>AAAAANHSTQESGFDYEGLIDSELQKKRLDKSYRYFNNINRLAKEFPLAHRQREADKVTVWCSNDYLALSKHPEVLDAMHKTIDKYGCGAGGTRNIAGHNIPTLNLEAELATLHKKEGALVFSSCYVANDAVLSLLGQKMKDLVIFSDELNHASMIVGIKHANVKKHIFKHNDLNELEQLLQSYPKSVPKLIAFESVYSMAGSVADIEKICDLADKYGALTFLDEVHAVGLYGPHGAGVAEHCDFESHRASGIATPKTNDKGGAKTVMDRVDMITGTLGKSFGSVGGYVAASRKLIDWFRSFAPGFIFTTT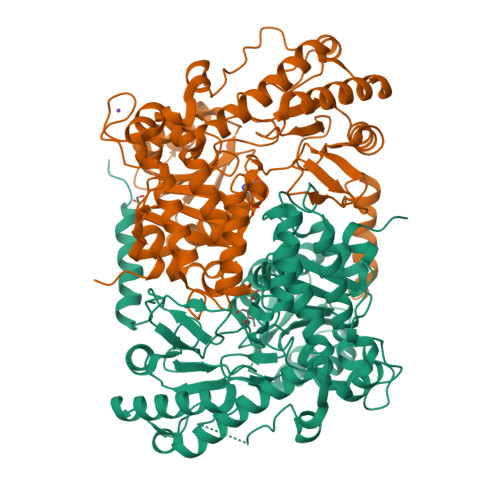LPPSVMAGATAAIRYQRCHIDLRTSQQKHTMYVKKAFHELGIPVIPNPSHIVPVLIGNADLAKQASDILINKHQIYVQAINFPTVARGTERLRITPTPGHTNDLSDILINAVDDVFNELQLPRVRDWESQGGLLGVGESGFVEESNLWTSSQLSLTNDDLNPNVRDPIVKQLEVSSGIKQ[2x]>PFTYSIEATRNLATTERCIQDIRNAPVRNRSTQFQLAQQNMLAYTFGEVIPGFASAGINGMDYRDVIGRPVENAVTEGTHFFRDDFRVDSNAKAKVAGDIFEIVSSAVMWNCAARWNSLMVGEGWRSQPRYSRPTLSPSPRRQVAVLNLPRSFDWVSLLVPESQEVIEEFRAGLRKDGLGLPTSTPDLAVVVLPEEFQNDEMWREEIAGLTRPNQILLSGAYQRLQGRVQPGEISLAVAFKRSLRSDRLYQPLYEANVMQLLLEGKLGAPKVEFEVHTLAPEGT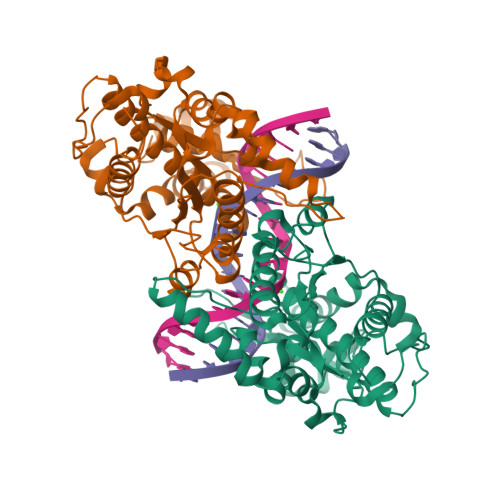NAFVTYEAASLYGLAEGRSAVHRAIRELYVPPTAADLARRFFAFLNERMELVNG[2x]>[2x]M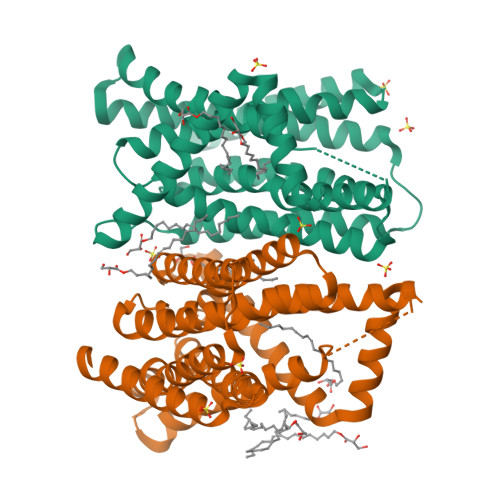NQPSSLAADLRGAWHAQAQSHPLITLGLAASAAGVVLLLVAGIVNALTGENRVHVGYAVLGGAAGFAATALGALMALGLRAISARTQDAMLGFAAGMMLAASAFSLILPGLDAAGTIVGPGPAAAAVVALGLGLGVLLMLGLDYFTPHEHERTGHQGPEAARVNRVWLFVLTIILHNLPEGMAIGVSFATGDLRIGLPLTSAIAIQDVPEGLAVALALRAVGLPIGRAVLVAVASGLMEPLGALVGVGISSGFALAYPISMGLAAGAMIFVVSHEVIPETHRNGHETTATVGLMAGFALMMFLDTALG Given the auxotrophic nature of pneumococci for certain amino acids, the Ami ABC transporter system, orchestrating oligopeptide uptake, becomes indispensable in host compartments lacking amino acids. The system comprises five exposed Oligopeptide Binding Proteins (OBPs) and four proteins building the ABC transporter channel. Crucially, SBPs determine the specificity of their respective transport systems, thereby governing the range of molecules capable of entering the cell. The five lipoproteins exhibit pairwise sequence identity of ~52–60% and share a very similar overall folding.

To evaluate AliB’s capacity to recognize diverse peptides, the protein was incubated with an excess of defined synthesized peptides (peptides 2, 3 and 4) that were previously reported to bind AliB. Specifically, crystal structures of AliB in complex with peptide 2 (AIQSEKARKHN), peptide 3 (PIVGGHEGAGV), and peptide 4 (VMVKGPGPGREST) were solved at resolutions of 2.29 Å, 1.66 Å and 1.49 Å, respectively. The three complexes obtained for AliB exhibited minimal backbone changes among them (rmsd ranging between 0.1 and 0.3 Å). In all three complexes, mirroring the observation in the AliD:peptide 1 complex, the amine N-terminus of the oligopeptide establishes a salt-bridge with an aspartic residue (D503) and van der Waals interactions with the neighboring tryptophan residue (W500). The region encompassing the first three residues of the ligands (AIQ in peptide 2, PIV in peptide 3 and VMV in peptide 4) folds in an antiparallel β-sheet-fashion with the β20 (G499, W500 and G501) from Lobe 1, and parallel β-sheet-like interactions with a loop of domain I (containing residues N52 and A54) on the opposite side. Beyond the third position, the recognition by AliB does not adhere to a conserved pattern, as each peptide adopts a distinct conformation within the substrate-binding cavity and establishes different interactions with the protein. For instance, in the case of peptide 2, the remaining portion of the oligopeptide immediately following the small β strand region, which exhibits a strong basic character (EKARKHN), adopts an α-helix conformation within the AliB cavity. This helical region finds stabilization through numerous H-bonds with the protein and is further reinforced by salt-bridge interactions involving the basic residues of the substrate interacting with the acidic residues of the protein (E351, E437, and D443). Regardless, the electrostatic potential of the AliB binding site exhibits a neutral character to facilitate interaction with the residue at position 2 through Van der Waals interactions, and a strongly acidic character after position 4, enabling the stabilization of basic residues of the oligopeptides through salt-bridge interactions.

> NSSTASKTYNYVYSSDPSSLNYLAENRAATSDIVANLVDGLLENDQYGNIIPSLAEDWTVSQDGLTYTYKLRKDAKWFTSEGEEYAPVTAQDFVTGLQYAADKKSEALYLVQDSVAGLDDYITGKTSDFSTVGVKALDDQTVQYTLVKPELYWNSKTLATILFPVNADFLKSKGDDFGKADPSSILYNGPFLMKALVSKSAIEYKKNPNYWDAKNVFVDDVKLTYYDGSDQESLERNFTAGAYTTARLFPNSSSYEGIKEKYKNNIIYSMQNSTSYFFNFNLDRKSYNYTSKTSDIEKKSTQEAVLNKNFRQAINFAFDRTSYGAQSEGKEGATKILRNLVVPPNFVSIKGKDFGEVVASKMVNYGKEWQGINFADGQDPYYNPEKAKAKFAEAKKELEAKGVQFPIHLDKTVEVTDKVGIQGVSSIKQSIESVLGSDNVVIDIQQLTSDEFDSSGYFAQTAAQKDYDLYHGGWGPDYQDPSTYLDIFNTNSGGFLQNLGLEPGEANDKAKAVGLDVYTQMLEEANKEQDPAKRYEKYADIQAWLIDSSLVLPSVSRGGTPSLRRTVPFAAAYGLTGTKGVESYKYLKVQDKIVTTDEYAKAREKWLKEKEESNKKAQEELAKHVK;> AIQSEKARKHN2-methoxyethyl propan-2-yl 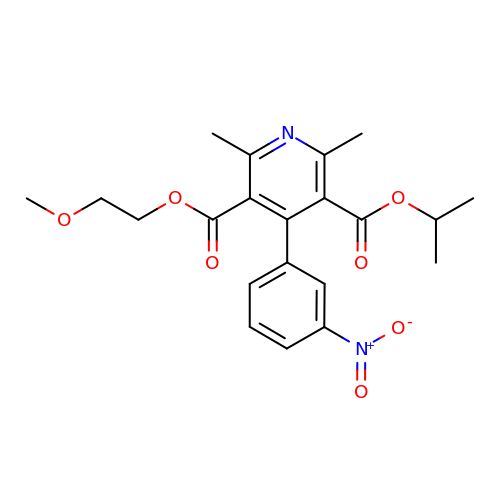2,6-dimethyl-4-(3-nitrophenyl)pyridine-3,5-dicarboxylate | C21 H24 N2 O7 | SJJUCKCPGPCJQM-UHFFFAOYSA-N>[2x]MVMTIATPLKAQPKASHFIDGDYVEDNTGTPFESIFPATGEMIAKLHAATPAIVERAIASAKRAQKEWAAMSPMARGRILKRAADIMRERNDALSTLETLDTGKPIQETIVADPTSGADAFEFFGGIAPSALNGDYIPLGGDFAYTKRVPLGVCVGIGAWNYPQQIACWKAAPALVAGNAMVFKPSENTPLGALKIAEILIEAGLPKGLFNVIQG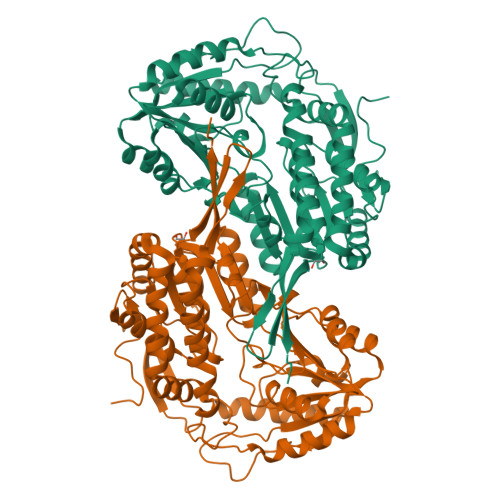DRDTGPLLVNHPDVAKVSLTGSVPTGRKVAAAAAGHLKHVTMELGGKSPMIVFDDADIESAVGGAMLGNFYSSGQVCSNGTRVFVQKKAKARFLENLKRRTEAMILGDPLDYATHLGPLVSKAQQEKVLSYIEKGKAEGATLITGGGIPNNVAGEGAYVQPTVFADVTDDMTIAREEIFGPVMCVLDFDDEDEVLARANATEFGLAGGVFTADLARAHRVVDGLEAGTLWINTYNLCPVEIPFGGSKQSGFGRENSAAALEHYSELKTVYVSTGKVDAPYAENLYFQSHHHHHHWSHPQFEK> MSTFIRGPICGTDNCPSRLWRIIDGRRTCQYGHVMEGDVEFNDDEDDLNGLGAGVITRRLNLTTNATGSFQSSQLTNSQLLQQQQRQSHKKFKKLIGHEAKLLFLKSFQFILKRQIRWLITEMRFPKEFEHVAKIIWLKILKTINDQPQEELKLQLHMTSTISILYLASTHLSLPVYTCDYIKWICTAKMPYFQASEILPKSWRIQLPNYYVSILEGSISPFNGQLYNKIALTCGMIHFKEFFNSEISCQGLLLKLVMQCALPPEFYFYTKQVIEFEETDIRNLTLWERTDERHTGRVSNHAELRVLSYFMLTINWMLSFDRDRQYPLKWILSLTESLTQRTTTSESIGRNIVKVVYPDKPTSSDYFQWSEEETLEFLKWMEKQFLPTQTKSLHNENGSMEMTIDQKIARRKLYKIFPLDREANHDGEFNDSTHQLTFIEDLQERYAKQTPFFESNKIRDSLNYQEANPPARKEAI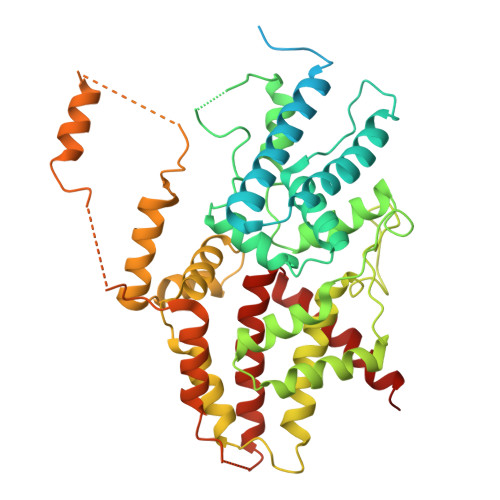GRLLTHIASQLLVDFAISKEQLKDCISRIKNACLHRMN> GPMTDQAFVTLTTNDAYAKGALVLGSSLKQHRTTRRLVVLATPQVSDSM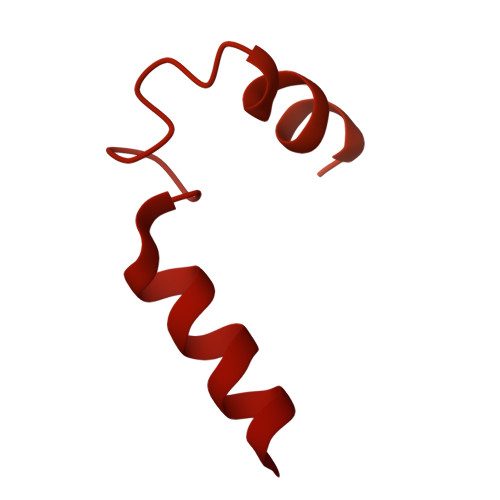RKVLETVFDEVIMVDVLDSGDSAHLTLMKRPELGVTLTKLHCWSLTQYSKCVFMDADTLVLANIDDLFDREELSAAPDPGWPDCFNSGVFVYQPSVETYNQLLHLASEQGSFDGGDQGILNTFFSSWATTDIRKHLPFIYNLSSISIFSYLPAFKVFGASAKVVHFLGRVKPWNYTYDPKTKSVKSEAHDPNMTHPEFLILWWNIFTTNVLPLLQQFGLVKDTCSYVNVLSDLVYTLAFSCGFCRKEDVSGAISHLSLGEIPAMAQPFVSSEERKERWEQGQADYMGADSFDNIKRKLDTYLQ>MAVPQFHRPSTVTTDSVRALGMRGLVLATNNSQFIMDNNHPHPQGTQGAVREFLRGQAAALTDLGLAHANNTFTPQPMFAGDAPAAWLRPAFGLRRTYSPFVVREPSTPGTP[15x];>MAAPNRDPPGYRYAAAMVPTGSLLSTIEVASHRRLFDFFSRVRSDANSLYDVEFDALLGSYCNTLSLVRFLELGLSVACVCTKFPELAYMNEGRVQFEVHQPLIARDGPHPIEQPTHNYMTKIIDRRALNAAFSLATEAIALLTGEALDGTGIGAHRQLRAIQQLARNVQAVLGAFERGTADQMLHVLLEKAPPLALLLPMQRYLDNGRLATRVARATLVAELKRSFCETSFFLGKAGHRREAVEAWLVDLTTATQPSVAVPRLTHADTRGRPVDGVLVTTAPIKQRLLQSFLKVEDTEADVPVTYGEMVLNGANLVTALVMGKAVRSLDDVGRHLLEMQEEQLDLNRQTLDELESAPQTTRVRADLVSIGEKLVFLEALEKRIYAATNVPYPLVGAMDLTFVLPLGLFNPVMERFAAHAGDLVPAPGHPDPRAFPPRQLFFWGKDRQVLRLSLEHAIGTVCHPSLMNVDAAVGGLNRDPVEAANPYGAYVAAPAGPAADMQQLFLNAWGQRLAHGRVRWVAEGQMTPEQFMQPDNANLALELHPAFDFFVGVADVELPGGDVPPAGPGEIQATWRVVNGNLPLALCPAAFRDARGLELGVGRHAMAPATIAAVRGAFDDRNYPAVFYLLQAAIHGSEHVFCALARLVVQCITSYWNNTRCAAFVNDYSLVSYVVTYLGGDLPEECMAVYRDLVAHVEALAQLVDDFTLTGPELGGQAQAELNHLMRDPALLPPLVWDCDALMRRAALDRHRDCRVSAGGHDPVYAAACNVATADFNRNDGQLLHNTQARAADAADDRPHRGADWTVHHKIYYYVMVPAFSRGRCCTAGVRFDRVYATLQNMVVPEIAPGEECPSDPVTDPAHPLHPANLVANTVNAMFHNGRVVVDGPAMLTLQVLAHNMAERTTALLCSAAPDAGANTASTTNMRIFDGALHAGILLMAPQHLDHTIQNGDYFYPLPVHALFAGADHVANAPNFPPALRDLSRQVPLVPPALGANYFSSIRQPVVQHVRESAAGENALTYALMAGYFKISPVALHHQLKTGLHPGFGFTVVRQDRFVTENVLFSERASEAYFLGQLQVARHETGGGVNFTLTQPRGNVDLGVGYTAVVATATVRNPVTDMGNLPQNFYLGRGAPPLLDNAAAVYLRNAVVAGNRLGPAQPVPVFGCAQVPRRAGMDHGQDAVCEFIATPVSTDVNYFRRPCNPRGRAAGGVYAGDKEGDVTALMYDHGQSDPSRAFAATANPWASQRFSYGDLLYNGAYHLNGASPVLSPCFKFFTSADIAAKHRCLERLIVETGSAVSTATAASDVQFKRPPGCRELVEDPCGLFQEAYPLTCASDPALLRSARNGEAHARETHFAQYLVYDASPLKGLAL[16x];>MKTNPLPATPSVWGGSTVELPPTTRDTAGQGLLRRVLRPPISRRDGPGLPRGSGPRRAASTLWLLGLDGTDAPPGALTPNDDTEQALDKILRGTMRGGAALIGSPRHHLTRQVILTDLCQPNADRAGTLLLALRHPADLPHLAHQRAPPGRQTERLGEAWGQLMEATALGSGRAESGCTRAGLVSFNFLVAACAASYDARDAADAVRAHVTANYRGTRVGARLDRFSECLRAMVHTHVFPHEVMRFFGGLVSWVTQDELASVTAVCAGPQEAAHTGHPGRPRSAVILPACAFVDLDAELGLGGPGAAFLYLVFTYRQRRDQELCCVYVIKSQLPPRGLEPALERLFGRLRITNTIHGTEDMTPPAPNRNPDFPLAGLAANPQTPRCSAGQVTNPQFADRLYRWQPDLRGRPTARTCTYAAFAELGMMPEDSPRCLHRTERFGAVSVPVVILEGVVWRPGEWRACA[5x];>[10x]MLADGFETDIAIPSGISRPDAAALQRCEGRVVFLPTIRRQLTLADVAHESFVSGGVSPDTLGLLLAYRRRFPAVITRVLPTRIVACPLDVGLTHAGTVNLRNTSPVDLCNGDPISLVPPVFEGQATDVRLDSLDLTLRFPVPLPSPLAREIVARLVARGIRDLNPSPRNPGGLPDLNVLYYNGSRLSLLADVQQLGPVNAELRSLVLNMVYSITEGTTIILTLIPRLFALSAQDGYVNALLQMQSVTREAAQLIHPEAPALMQDGERRLPLYEALVAWLTHAGQLGDTLALAPVVRVCTFDGAAVVRSGDMAPVIRYP;> MNAHLANEVQYDLGHGPGRPSSLVHVIISSECLAAAGIPLAALMRGRPGLGTAANFQVEIQTRAHATGDCTPWCTAFAAYVPADAVGELLAPVVPAHPGLLPRASSAGGLFVSLPVVCDAQGVYDPYAVAALRLAWGSGASCARVILFSYDELVPPNTRYAADSTRIMRVCRHLCRYVALLGAAAPPAAKEAAAHLSMGLGESASPRPQPLARPHAGAPADPPIVGASDPPISPEEQLTAPGGDTTAAQDVSIAQENEEILALVQRAVQDVTRRHPVRARTGRAACGVASGLRQGALVHQAVSGGAMGAADADAVLAGLEPPGGGRFVAPAPHGPGGEDILNDVLTLTPGTAKPRSLVEWLDRGWEALAGGDRPDWLWSRRSISVVLRHHYGTKQRFVVVSYENSVAWGGRRARPPLLSSALATALTEACAAERVVRPHQLSPAGQAELLLRFPALEVPLRHPRPVLPPFDIAAEVAFTARIHLACLRALGQAIRAALQGGPRISQRLRYDFGPDQRAWLGEVTRRFPILLENLMRAVEGTAPDAFFHTAYALAVLAHLGGRGGRGRRVVPLGDDLPARFADSDGHYVFDYYSTSGDTLRLNNRPIAVAMDGDVSKREQSKCRFMEAVPSTAPRRVCEQYLPGESYAYLCLGFNRRLCGIVVFPGGFAFTINIAAYLSLSDPVARAAVLRFCRKVSSGNGRSR;>MDPYCPFDALDVWEHRRFIVADSRNFITPEFPRDFWMSPVFNLPRETAAEQVVVLQAQRTAAAAALENAAMQAAELPVDIERRLRPIERNVHEIAGALEALETAAAAAEEADAARGDEPAGGGDGGAPPGLAVAEMEVQIVRNDPPLRYDTNLPVDLLHMVYAGRGATGSSGVVFGTWYRTIQDRTITDFPLTTRSADFRDGRMSKTFMTALVLSLQACGRLYVGQRHYSAFECAVLCLYLLYRNTHGAADDSDRAPVTFGDLLGRLPRYLACLAAVIGTEGGRPQYRYRDDKLPKTQFAAGGGRYEHGALASHIVIATLMHHGVLPAAPGDVPRDASTHVNPDGVAHHDDINRAAAAFLSRGHNLFLWEDQTLLRATANTITALGVIQRLLANGNVYADRLNNRLQLGMLIPGAVPSEAIARGASGSDSGAIKSGDNNLEALCANYVLPLYRADPAVELTQLFPGLAALCLDAQAGRPVGSTRRVVDMSSGARQAALVRLTALELINRTRTNPTPVGEVIHAHDALAIQYEQGLGLLAQQARIGLGSNTKRFSAFNVSSDYDMLYFLCLGFIPQYLSAV[2x];>[2x]MIAGTPPHSTMERGGDRDIVVTGARNQFAPDLEPGGSVSCMRSSLSFLSLIFDVGPRDVLSAEAIEGCLVEGGEWTRATAGPGPPRMCSIVELPNFLEYPGARGGLRCVFSRVYGEVGFFGEPAAGLLETQCPAHTFFAGPWALRPLSYTLLTIGPLGMGLFRDGDTAYLFDPHGLPEGTPAFIAKVRAGDMYPYLTYYTRDRPDVRWAGAMVFFVPSGPEPAAPADLTAAALHLYGASETYLQDEAFSERRVAITHPLRGEIAGLGEPCVGVGPREGVGGPGPHPPTAAQSPPPTRARRDDRASETSRGTAGPSAKPEAKRPNRAPDDVWAVALKGTPPTDPPSADPPSADPPSAIPPPPPSAPKTPAAEAAEEDDDDMRVLEMGVVPVGRHRARYSAGLPKRRRPTWTPPSSVEDLTSGEKTKRSAPPAKTKKKSTPKGKTPVGAAVPASVPEPVLASAPPDPAGPPVAEAGEDDGPTVPASSQALEALKTRRSPEPPGADLAQLFEAHPNVAATAVKFTACSAALAREVAACSRLTISALRSPYPASPGLLELCVIFFFERVLAFLIENGARTHTQAGVAGPAAALLEFTLNMLPWKTAVGDFLASTRLSLADVAAHLPLVQHVLDENSLIGRLALAKLILVARDVIRETDAFYGELADLELQLRAAPPANLYTRLGEWLLERSQAHPDTLFAPATPTHPEPLLYRVQALAKFARGEEIRVEAEDRQMREALDALARGVDAVSQHAGPLGVMPAPAGAAPQGAPRPPPLGPEAVQVRLEEVRTQARRAIEGAVKEYFYRGAVYSAKALQASDNNDRRFHVASAAVVPVVQLLESLPVFDQHTRDIAQRAAIPAPPPIATSPTAILLRDLIQRGQTLDAPEDLAAWLSVLTDAANQGLIERKPLDELARSIRDINDQQARRSSGLAELRRFDALDAALGQQLDSDAAFVPAPGASPYPDDGGLSPEATRMAEEALRQARAMDAAKLTAELAPDARARLRERARSLEAMLEGARERAKVARDAREKFLHKLQGVLRPLPDFVGLKACPAVLATLRASLPAGWSDLPEAVRGAPPEVTAALRADMWGLLGQYRDALEHPTPDTATALSGLHPSFVVVLKNLFADAPETPFLLQFFADHAPIIAHAVSNAINAGSAAVATADPASTVDAAVRAHRVLVDAVTALGAAASDPASPLAFLAAMADSAAGYVKATRLALDARVAIAQLTTLGSAAADLVVQVRRAANQPEGEHASLIQAATRATTGARESLAGHEGRFGGLLHAEGTAGDHSPSGRALQELGKVIGATRRRADELEAATADLREKMAAQRARSSHERWAADVEAVLDRVESGAEFDVVELRRLQALAGTHGYNPRDFRKRAEQALGTNAKAVTLALETALAFNPYTPENQRHPMLPPLAAIHRIDWSAAFGAAADTYADMFRVDTEPLARLLRLAGGLLERAQANDGFIDYHEAVLHLSEDLGGVPALRQYVPFFQKGYAEYVDIRDRLDALRADARRAIGSVALDLAAAAEEISAVRNDPAAAAELVRAGVTLPCPSEDALVACVAALERVDQSPVKDTAYADYVAFVTRQDLADTKDAVVRAKQQRAEATERVTAGLREVLAARERRAQLEAEGLANLKTLLKVVAVPATVAKTLDQARSAEEIADQVEILVDQTEKARELDVQAVAWLEHAQRTFETHPLSAASGDGPGLLTRQGARLQALFDTRRRVEALRRSLEEAEAEWDEVWGRFGRVRGGAWKSPEGFRAACEQLRALQDTTNTVSGLRAQRDYERLPAKYQGVLGAKSAERAGAVEELGGRVAQHADLSARLRDEVVPRVAWEMNFDTLGGLLAEFDAVAGDLAPWAVEEFRGARELIQRRMGLYSAYAKATGQTGAGAAAAPAPLLVDLRALDARARASAPPGQEADPQMLRRRGEAYLRVSGGPGPLVLREATSTLDRPFAPSFLVPDGTPLQYALCFPAVTDKLGALLMCPEAACIRPPLPTDTLES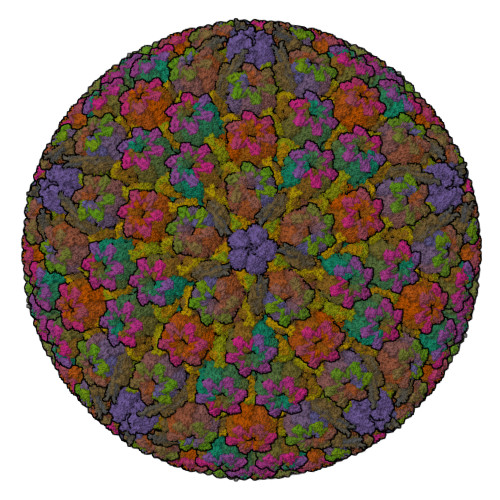ASTVTAMYVLTVINRLQLALSDAQAANFQLFGRFVRHRQARWGASMDAAAELYVALVATTLTREFGCRWAQLEWGGDAAAPGPPLGPQSSTRHRVSFNENDVLVALVASSPEHIYTFWRLDLVRQHEYMHLTLPRAFQNAADSMLFVQRLTPHPDARIRVLPAFSAGGPPTRGLMFGTRLADWRRGKLSETDPLAPWRSVPELGTERGAALGKLSPAQALAAVSVLGRMCLPSTALVALWTCMFPDDYTEYDSFDALLTARLESGQTLSPSGGREASPPAPPNALYRPTGQHVAVPAAATHRTPAARVTAMDLVLAAVLLGAPVVVALRNTTAFSRESELELCLTLFDSRARGPDAALRDAVSSDIETWAVRLLHADLNPIENACLAAQLPRLSALIAERPLARGPPCLVLVDISMTPVAVLWENPDPPGPPDVRFVGSEATEELPFVAGGEDVLAASATDEDPFLARAILGRPFDASLLSGELFPGHPVYQRAPDDQSPSVPNPTPGPVDLVGAEGSLGPGSLAPTLFTDATPGEPVPPRMWAWIHGLEELASDDSGGPAPLLAPDPLSPTADQSVPTSQCAPRPPGPAVTAREARPGVPAESTRPAPVGPRDDFRRLPSPQSSPAPPDATAPRPPASSRASAASSSGSRARRHRRARSLARATQASATTQGWRPPALPDTVAPVTDFARPPAPPKPPEPAPHALVSGVPLPLGPQAAGQASPALPIDPVPPPVATGTVLPGGENRRPPLTSGPAPTPPRVPVGGPQRRLTRPAVASLSESRESLPSPWDPADPTAPVLGRNPAEPTSSSPAGPSPPPPAVQPVAPPPTSGPPPTYLTLEGGVAPGGPVSRRPTTRQPVATPTTSARPRGHLTVSRLSAPQPQPQPQPQPQPQPQPQPQPQPQPQPQPQPQPQPQPQPQPQPQPQPQPQPQPQPQPQPQPQPQPQPQPQNGHVAPGEYPAVRFRAPQNRPSVPASASSTNPRTGSSLSGVSSWASSLALHIDATPPPVSLLQTLYVSDDEDSDATSLFLSDSEAEALDPLPGEPHSPITNEPFSALSADDSQEVTRLQFGPPPVSANAVLSRRYVQRTGRSALAVLIRACYRLQQQLQRTRRALLHHSDAVLTSLHHVRMLLG> SWRLKDETYSYDGKLGADLKEEGKQVDLTLWSPSADKVSVVVYDKNDPDKVVGTVALEKGERGTWKQTLDSTNKLGITDFTGYYYQYQIERQGKTVLALDPYAKSLAAWNSDDSKIDDAHKVAKAAFVDPAKLGPQDLTYGKIHNFKTREDAVIYEAHVRDFTSDPAIAKDLTKPFGTFEAFIEKLDYLKDLGVTHIQLLPVLSYYFVNELKNHERLSDYASSNSNYNWGYDPQNYFSLTGMYSSDPKNPEKRIAEFKNLINEIHKRGMGAILDVVYNHTAKVDLFEDLEPNYYHFMDADGTPRTSFGGGRLGTTHHMTKRLLIDSIKYLVDTYKVDGFRFDMMGDHDAASIEEAYKAARALNPNLIMLGEGWRTYAGDENMPTKAADQDWMKHTDTVAVFSDDIRNNLKSGYPNEGQPAFITGGKRDVNTIFKNLIAQPTNFEADSPGDVIQYIAAHDNLTLFDIIAQSIKKDPSKAENYAEIHRRLRLGNLMVLTAQGTPFIHSGQEYGRTKQFRNPAYRTPVAEDKVPNKSHLLRDKDGNPFDYPYFIHDSYDSSDAVNKFDWTKATDGKAYPENVKSRDYMKGLIALRQSTDAFRLKSLQDIKDRVHLITVPGQNGVEKEDVVIGYQITAPNGDIYAVFVNADEKAREFNLGTAFAHLRNAEVLADEN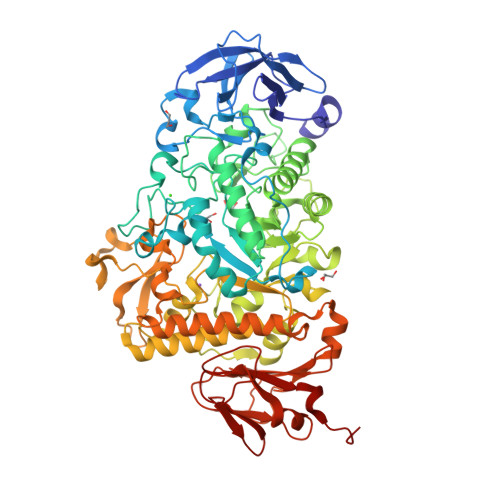QAGPVGIANPKGLEWTEKGLKLNALTATVLRVSQNGTSHEST>[3x]GSHMACVNEPSPKLQKLDRNGIHGDSSPSPFFKVKKLS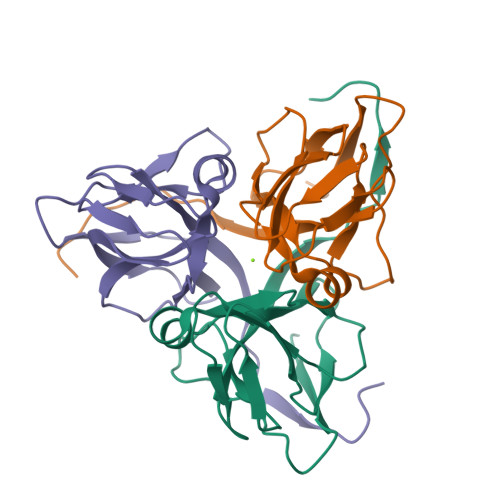EKAVIPTRGSPLSAGYDLSSAVDSKVPARGKALIPTDLSIAVPEGTYARIAPRSGLAWKHSIDVGAGVIDADYRGPVGVILFNHSDADFEVKFGDRIAQLIIEKIVTPDVVEVDDLDETVRGDGGFGSTGV> VVGGTDADEGEWPWQVSLHALGQGHICGASLISPNWLVSAAHCYIDDRGFRYSDPTQWTAFLGLHDQSQRSAPGVQERRLKRIISHPFFNDFTFDYDIALLELEKPAEY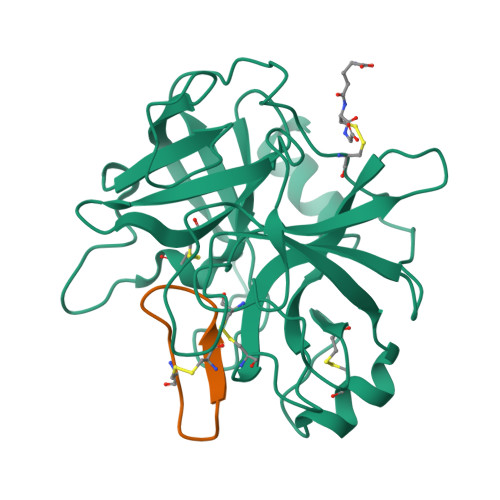SSMVRPICLPDASHVFPAGKAIWVTGWGHTQYGGTGALILQKGEIRVIQQTTCENLLPQQITPRMMCVGFLSGGVDSCQGDSGGPLSSVEADGRIFQAGVVSWGDGCAQRNKPGVYTRLPLFRDWIKENTGV;> GRCTKSIPPICFPD>DGTSQLAELVDAAAERLEVADPVAAFKWRAQLPIEDSGRVEQQLAKLGE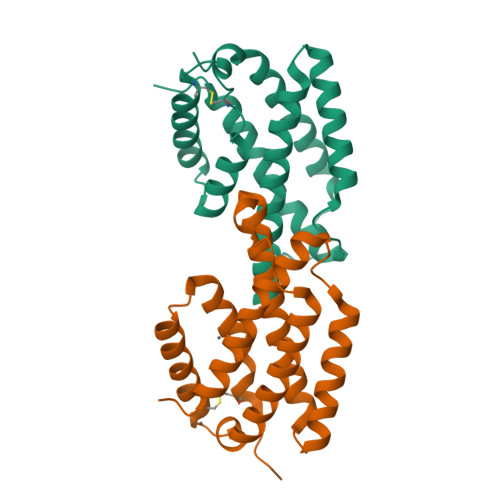DARSQHIDPDYVTRVFDDQIRATEAIEYSRFSDWKLNPASAPPEPPDLSASRSAIDSLNNRMLSQIWSHWSLLSAPSCAAQLDRAKRDIVRSRHLDSLYQRALTTATQSYCQALPPA[2x]> MAHHHHHHMSNSAMSVVILAAGKGTRMYSDLPKVLHTLAGKPMVQHVIDAANDLGACAVHLVYGHGGDLLRQTLHEDNLNWVLQAEQLGTGHAMQQAAPFFNDDEDILMLYGDVPLISVETLQRLRAAKPQGGIGLLTVKLDDPTGYGRITRENGQVTGIVEHKDASEAQRQIQEINTGILIAGGADLKRWLAKLTNNNAQGEYYITDIIAMAHQEGHQIVAVHPQRLSEVEGVNNRLQLARLERVYQAEQAEKLLLAGVMLRDPARFDLRGTLQHGRDVEIDTNVILEGNVVLGDRVKIGAGCVIKNSTIGDDCEISPYSVVEDAQLQAACTIGPFARLRPGAELLEGAHVGNFVEMKKARLGK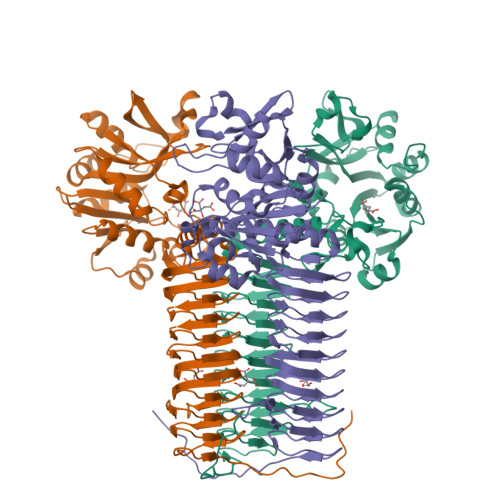GSKAGHLTYLGDAEIGDNVNIGAGTITCNYDGANKHKTIIGDDVFVGSDTQLVAPVTVGNGVTIAAGTTVTRNIADNELVLSRVPQVHKQGWQRPVKKK6-{(3R)-3-[(4-tert-butylbenzoyl)amino]piperidin-1-yl}-2-{[4-(morpholin-4-ylcarbonyl)phenyl]amino}pyridine-3-carboxamide | C33 H40 N6 O4 | 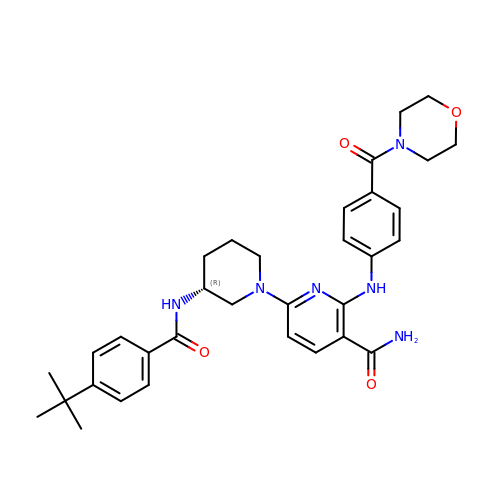HIYRPMYMGBHLMP-AREMUKBSSA-N> MGSSHHHHHHSQDPKISDVVVELFREAAIYLPEDVKNALEEAYKKESSEISKNTLKAIIENNKIAEETQVPLCQDTGVPIVFLKIGKNINSSEIMKIIEEIKEGVKKATEEVPLRPNVVHPLTRENFKTNVGLNSPFINIEFDESLDREIEIIAFPKGAGSENMSALKMLKPSDGIEGIKNFVLETIANAGGKPCPPIVVGIGIGGTADVALKLAKKALLRKIGERHRDKEIANLEKELLEKINSLGIGAMGLGGDITALDVFIEIAGCHTASLPVGICIQCWADRRAIKRIKLDAKL;> MEYTFNKLTKKDVKKLKVGDIVYLNGKIYTARDEAHLK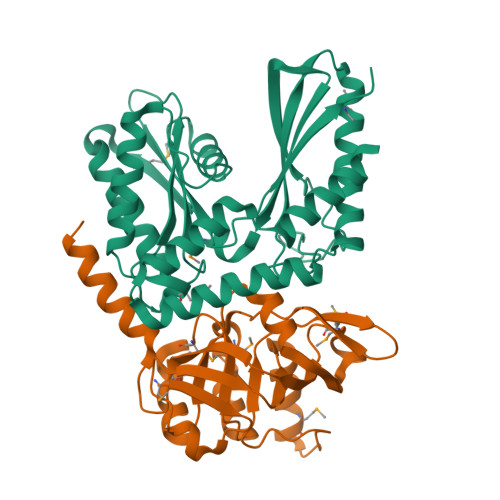IIEMLKSNEKLPFDLNESIIYHAGPIMKKVNDSWVCVSIGPTTSARMNDVEEEFIKLTNISAIVGKGGMKKELLKTFEDYGVVYLAAPGGCAALLANSVKRVDNVYFLDELGMPEAVWELEVNNFGPLIVAMDSHGNSIYEEVNKKVYEKLNELIGL>MIIKPRIRGFICTTTHPVGCEQNVKEQIALTKAQGPIANAPKRVLVVGSSSGYGLSSRITAAFGGGASTIGVFFEKAGTEKKPGTAGWYNSAAFDKFAKEEGLYSKSLNGDAFSNEAKQKTIDLIKEDLGQIDMVVYSLASPVRKMPETGEVIRSSLKPIGETYTATAVDTNKDAIIEASVEPATEQEIKDTVTVMGGEDWELWINALSEAGV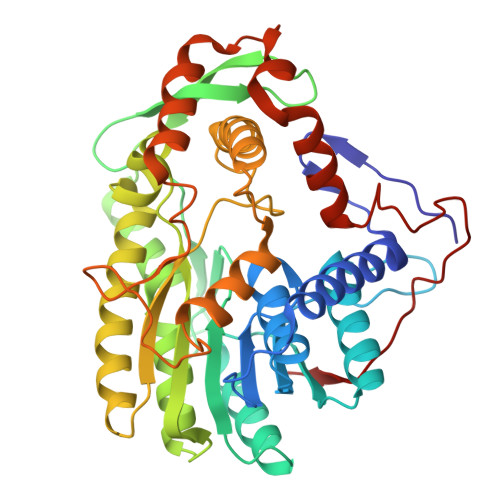LADGCKTVAYSYIGTELTWPIYWDGALGQAKMDLDRAATALNEKLSATGGTANVAVLKSVVTQASSAIPVMPLYIAMVFKKMREEGVHEGCQEQILRMFSQRLYKADGSAAEVDEKNRLRLDDWELREDIQQHCRDLWPQVTTENLKDLTDYVEYKEEFLKLFGFGVDGVDYDADVNPEVNFDVADI[2x]COMPASS is a multi-subunit complex in which the catalytic unit, SET1, is required for H3K4 methylation. An important subunit known to regulate SET1 methyltransferase activity is the CxxC zinc finger protein 1 (Cfp1). Cfp1 binds to COMPASS and is critical to maintain high level of H3K4me3 in cells but the mechanisms underlying its stimulatory activity is poorly understood. Finally, the ability of Cfp1 to associate with SET1A/B and unmethylated CpG islands increases the retention of COMPASS to chromatin.

To confirm this, we solved the crystal structure of Cfp1 RID at 2.3 Å. As defined by the electron density map, Cfp1 RID domain comprises residues 322–508, with one molecule in the asymmetric unit. This region of Cfp1 forms a three α-helix bundle with one Zn2+ atom binding site. The metal binding site is formed by two loops (referred to as L1 and L2). L1 is located at the C-terminus of α1 while L2 is located between α2 and α3. In L1, one metal coordinating residue, C378, is found in the conserved motif XCGΦ (also referred to as motif I) while in L2, C451, H459, C456 are located in the motif CXXXK/RXXCXXHXXW (also referred to as motif II). Comparative analysis reveals that similar to ZC3H, ZC2HC, ZCCHC, THAP, ZMIZ and PARP-Type zinc fingers, CtCfp1 RID domain employs a trio of cysteine residues and the side chain of a histidine to coordinate the zinc ion. However, in stark contrast to ZC3H and THAP, the residues forming the first cluster in CtCfp1 RID ZnF are separated by ∼80 residues; a distance that exceeds all the other zinc binding domain reported to date. Therefore, these observations suggest that the ZnF of Cfp1 RID is a novel type of ZnF. However, mutation of the residues forming both motifs and Tyr380 severely impede the binding of RbBP5 to Cfp1.

> ALTPEEYAELTASAETRSKLSEQIALCRQMLQLIELAIARREAAIAAGIPGITKDICGYDTRLDTVGAAHQFSLFLQSPQGQSIFSTRSLDNPPYVTTTIKNPEDDTPAATSSNSAETAAGQDPRTAGMCLRKKCKPHNGWGALLTKTVRHDIRELALQIRELLEAEQRVRDGAAGRFMRRMKERNEVIAIEEDEDDDEHGNGFLREEKLGHKRSDGDRMDLD> HKCDITLQEIIKTLNSLTEQKTLCTELTVTDIFAASKNTTEKETFCRAATVLRQFYSHHEKDTRCLGATAQQFHRHKQLIRFLKRLDRNLWGLAGLNSCPVKEANQSTLENFLERLKTIMREKYSKCSS;> ADPFKVLQEPTCVSDYMSISTCEWKMNGPTQCSTELRLLYQLVFLLSEAHTCIPENNGGAGCVCHLLMDDVVSADQYTLDLWAGQQLLWKGSFKPSEHVKPRAPGNLTVHTQVSDTLLLTWSNPYPPDNYLYNHLTYAVNIWSENDPADFRIYQVTYLEPSLRIAASTLKSGISYRARVRAWAQCYNTTWSEWSPSTKWHNSYRE;> TETQPPVTNLSVSVENLCTVIWTWNPPEGASSNCSLWYFSHFGDKQDKKIAPETRRSIEVPLNERICL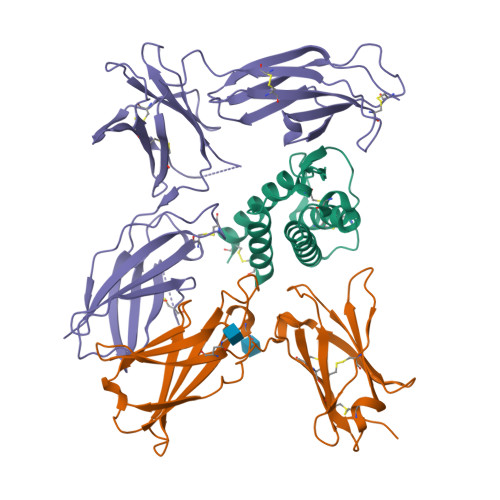QVGSQCSTNESEKPSILVEKCISPPEGDPESAVTELQCIWHNLSYMKCSWLPGRNTSPDTNYTLYYWHRSLEKIHQCENIFREGQYFGCSFDLTKVKDSSFEQHSVQIMVKDNAGKIKPSFNIVPLTSRVKPDPPHIKNLSFHNDDLYVQWENPQNFISRCLFYEVEVNNSQTETHNVFYVQEAKCENPEFERNVENTSCFMVPGVLPDTLNTVRIRVKTNKLCYEDDKLWSNWSQEMSIGKKRNS>[8x]MPHRFKVYNYMSPTFCDHCGSLLWGLVKQGLKCEDCGMNVHHKCREKVANLCG

Diacylglycerol (DAG) is a versatile lipid whose 1,2-sn-stereoisomer serves both as second messenger in signal transduction pathways that control vital cellular processes, and as metabolic precursor for downstream signaling lipids such as phosphatidic acid. Effector proteins translocate to available DAG pools in the membranes by using conserved homology 1 (C1) domains as DAG-sensing modules. PKCs define a central DAG-sensing node in intracellular phosphoinositide signaling pathways that regulate cell growth, differentiation, apoptosis, and motility. Herein, we report the high-resolution crystal structures of a C1 domain (C1B from PKCδ) complexed to DAG and to each of four potent PKC agonists that produce different biological readouts and that command intense therapeutic interest.

For structural studies, we formed the complex between the C1B domain of PKCδ (C1Bδ) and a synthetic DAG analog (di-octanoyl-sn-1,2-glycerol) in the presence of DPC micelles. The structure of the C1Bδ-DAG complex was refined to 1.75 Å with Rwork = 0.214 and Rfree = 0.246. The organization of the protein crystal lattice is unprecedented as it contains two distinct lipid-detergent micelles located at symmetry elements in the crystal. Each C1Bδ protein chain has a DAG molecule captured within a groove formed by its membrane-binding loop regions. DAG binds in the groove formed by the protein loops, β12 and β34 and can adopt two distinct binding modes: “sn-1” and “sn-2” 26. The “sn-1” mode is predominant in the crystal as it is observed in six of the eight C1Bδ chains. In both modes, the DAG glycerol and ester moieties are anchored to the C1Bδ binding groove by four hydrogen bonds. The fourth bond involves the amide hydrogen of Gly253 and it is this bond that defines the binding mode. In the “sn-1” position, the acceptor is the carbonyl oxygen O5 of the sn-1 ester group, whereas in the “sn-2” position the acceptor is the carbonyl oxygen O3 of the sn-2 ester group. A particularly important feature of the “sn-1” binding mode is the involvement of the alkoxy oxygen O2 of the sn-2 DAG chain in the hydrogen bond with the amide protons of the Gln257 sidechain.> MYGSTTARNLPSGKKQRIADLLSQIIETLDLTKTQYANIESAYNGVGTFLSEGDDPLLQDAVIYPQGSVRLNTTVKPKNEEQYDIDLICYLPHATQADYTGVISAIRQRLESHKTYKTLLSELPRGFRINYAGDYHLDITPGRDHTGTAHPGQPLWVVDAQTAWKESNPSGYAEWFESSASVQPLRTILVMDSASRVGTEALLPLPDSTDKKLLNHIVQILKRHRDEWAAEQDEVRQRCRPISVIITTLACHAYNHIIADRRAYDNDLDILLDVLELMPDFIVSTQGAIHVNNPHMPEENFAEKWNRSEQDEGPQRSEAFYQWHAAAQATFNTIAASVGEDNLFLSLEDSFGKTPVDVVRQRLMEHMQSAREQGSLHLDKKTGGLIATGLAGTAAQAGVPKNTFYGE;> MNNVVIRHHCK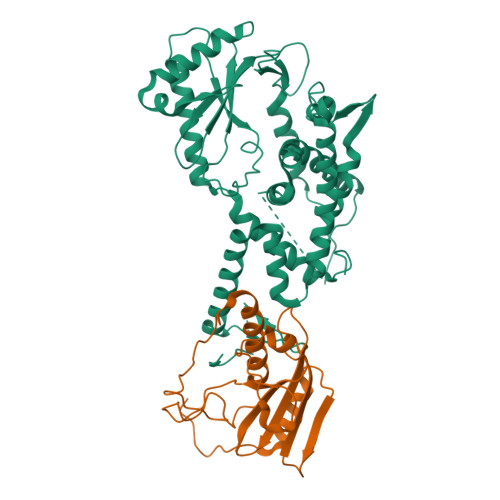PLTIAQQYRALKAGGPYERLRIIHHDRTLLWEGWLQPSLFSRRYKVAVRYSLGTPPICVVTEPDLFALAGTRAIPHLYPADKHIPGARLCLFLPRSQADDGLSEWRAQLKISDTLIPWASLWLFYFEQWLHTGHWEGGGKHPRPSEVKNER>[4x]MPGDEETLDLPAWNRVPDLTWGPHHRSAMASLDSEVREECLREDLKFYFMSPCEKYRARRQIPWKLGLQILKIVMVTTQLVRFGLSNQLVVAFKEDNTVAFKHLFLKGFSGVDEDDYSCSIYTQENTYESIFFAIKQYRHLKNISLATLGYGESEDNRTGLKVCKQH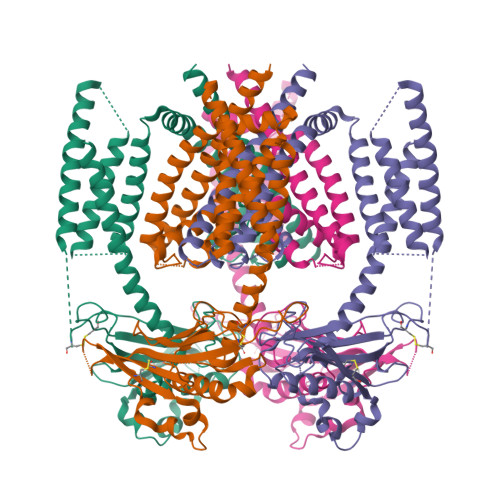YKTGAMFSSNETLNIDSDIETDCIHLDLQVLTTEPEDWAQTSFFRLDFYRLVQVDISFALKGIDLQAVHSREIPDCYLFQNTITFDNTAHSGKIKIYLNSEANIEECKNMNISGSTQRSTHYLLVFDVFVIMICLASLILCTRSIVLALRLRKRFLNFFLEKYKQRVCGADQWEFVNGWYVLVTISDLMTIIGSILKMEIKAKKLTNYDVCSILLGTSTLFVWVGVIRYLGYFQTYNVLILTMQASLPKVLRFCACAGMIYLGYTFCGWIVLGPYHEKFENLNIVAECLFSLVNGDDMFATFAQIQQKSILVWLFSRLYLYSFISLFIYMVLSLFIALITDSYHTIKKYQQ>[2x]SSLAPDYQRPAMPVPQQFSLSQNGLVNAADNYQNAGWRTFFVDNQVKTLISEALVNNRDLRMATLKVQEARAQYRLTDADRYPQLNGEGSGSWSGNLKGNTATTREFSTGLNASFDLDFFGRLKNMSEAERQNYLATEEAQRAVHILLVSNVAQSYFNQQLAYAQLQIAEETLRNYQQSYAFVEKQLLTGSSNVLALEQARGVIESTRSDIAKRQGELAQANNALQL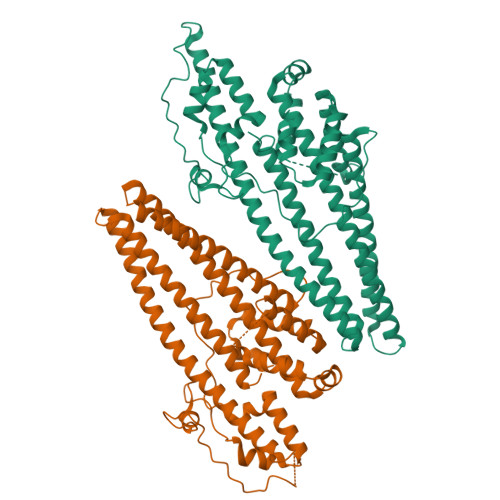LLGSYGKLPQAQTVNSDSLQSVKLPAGLSSQILLQRPDIMEAEHALMAANANIGAARAAFFPSISLTSGISTASSDLSSLFNASSGMWNFIPKIEIPIFNAGRNQANLDIAEIRQQQSVVNYEQKIQNAFKEVADALALRQSLNDQISAQQRYLASLQITLQRARALYQHGAVSYLEVLDAERSLFATRQTLLDLNYARQVNEISLYTALGGGHHHHHH>MRGEQGAAGARVLQFTNCRILRGGKLLREDLWVRGGRILDPEKLFFEERRVADERRDCGGRILAPGFIDVQINGGFGVDFSQATEDVGSGVALVARRILSHGVTSFCPTLVTSPPEVYHKVVPQIPVKSGGPHGAGVLGLHLEGPFISREKRGAHPEAHLRSFEADAFQDLLATYGPLDNVRIVTLAPELGRSHEVIRALTARGICVSLGHSVADLRAAEDAVWSGATFITHLFNAMLPFHHRDPGIVGLLTSDRLPAGRCIFYGMIADGTHTNPAALRIAHRAHPQGLVLVTDAIP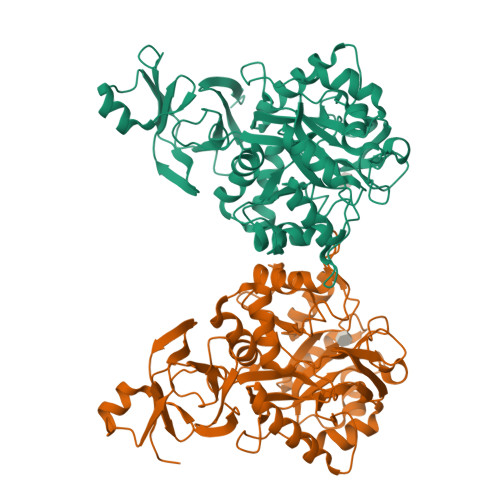ALGLGNGRHTLGQQEVEVDGLTAYVAGTKTLSGSIAPMDVCVRHFLQATGCSMESALEAASLHPAQLLGLEKSKGTLDFGADADFVVLDDSLHVQATYISGELVWQADAARQ[2x]> MKDQLSDEQKETIL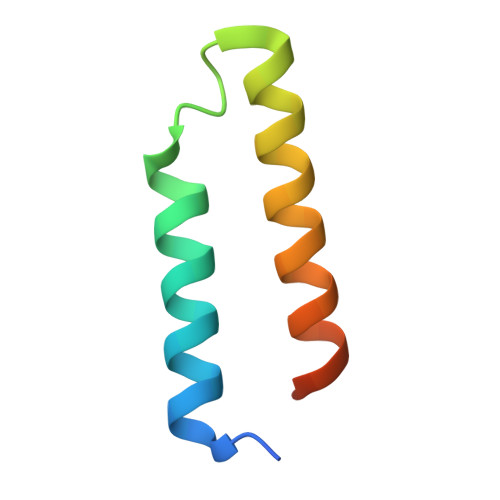KALNDAIEKGPWDKSNFLRVIGKKLIAIRDRFLKRIGAASQAK>[6x]GSSPNLRYPIADVSGGIGMSPNYRFRQSMWIGIVSYSGSGLNWRVQVNSDIFIVDDYIHICLPAFDGFSIADG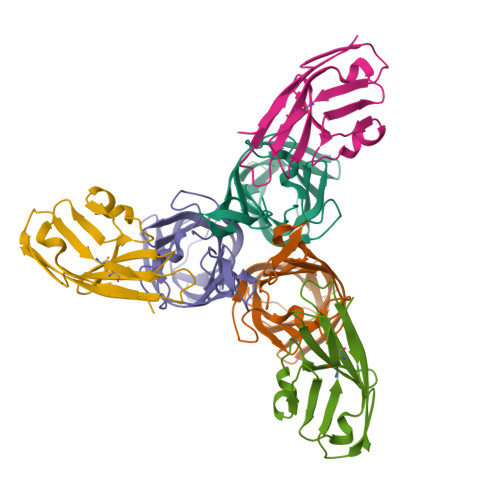GDLSLNFVTGLLPPLLTGDTEPAFHNDVVTYGAQTVAIGLSSGGTPQYMSKNLWVEQWQDGVLRLRVEGGGSITHSNSKWPAMTVSYPRSFT;>GSSVTVHSSEPEVRIPENNPVKLSCAYSGFSSPRVEWKFDQGDTTRLVCYNNKITASYEDRVTFLPTGITFKSVTREDTGTYTCMVSEEGGNSYGEVKVKLIVL[6x]Using a combination of biochemical and crystallographic methods we show that E. coli TldD and TldE interact to form a heterodimeric metalloprotease. TldD/E cleaves the N-terminal leader sequence from the modified MccB17 precursor peptide, to yield mature antibiotic, while it has no effect on the unmodified peptide. Both proteins are essential for the activity; however, only the TldD subunit forms a novel metal-containing active site within the hollow core of the heterodimer. Peptide substrates are bound in a sequence-independent manner through β sheet interactions with TldD and are likely cleaved via a thermolysin-type mechanism.

To explore the substrate binding site of the TldD/E heterodimer, wild-type or mutant (Glu263Ala) TldD/E was co-crystallized with a variety of peptides and peptide mimics, leading to four distinct ligand-bound complexes. Wild-type TldD/E crystals were grown in the presence of the peptide angiotensin II, and customized angiotensin II variant where the central (Tyr-Ile) peptide bond is replaced with a non-cleavable methylene bond, to yield two co-crystal structures with clear density for peptides where the carboxyl group of the C-terminal residue acts as a ligand to the catalytic zinc ion. However, the methylene bond variant gave density for a His-Pro-Phe peptide, i.e., the C-terminal portion of the added compound (hence WT-HPF); it was not clear whether the lack of clear density N-terminal to the His residue was due to a cleavage event, or simply that this region of the peptide was disordered. Using the standard nomenclature for protease active sites, these two ligands spanned subsites S4-S1 and S3-S1, respectively, occupying roughly half of the active site cleft.

>MGSSHHHHHHSQDPMSLNLVSEQLLAANGLKHQDLFAILGQLAERRLDYGDLYFQSSYHESWVLEDRIIKDGSYNIDQGVGVRAISGEKTGFAYADQISLLALEQSAQAARTIVRDSGDGKVQTLGAVEHSPLYTSVDPLQSMSREEKLDILRRVDKVAREADKRVQEVTASLSGVYELILVAATDGTLAADVRPLVRLSVSVLVEEDGKRERGASGGGGRFGYEFFLADLDGEVRADAWAKEAVRMALVNLSAVAAPAGTMPVVLGAGWPGVLLHEAVGHGLEGDFNRRGTSVFSGQVGELVASELCTVVDDGTMVDRRGSVAIDDEGTPGQYNVLIENGILKGYMQDKLNARLMGMTPTGNGRRESYAHLPMPRMTNTYMLPGKSTPQEIIESVEYGIYAPNFGGGQVDITSDKFVFSTSEAYLIENGKVTKPVKGATLIGSGIETMQQISMVGNDLKLDNGVGVCGKEGQSLPVGVGQPTLKVDNLTVGGTA[2x];>[2x]MALAMKVISQVEAQRKILEEAVSTALELASGKSDGAEVAVSKTTGISVSTRYGEVENVEFNSDGALGITVYHQNRKGSASSTDLSPQAIARTVQAALDIARYTSPDPCAGVADKELLAFDAPDLDLFHPAEVSPDEAIELAARAEQAALQADKRITNTEGGSFNSHYGVKVFGNSHGMLQGYCSTRHSLSSCVIAEENGDMERDYAYTIGRAMSDLQTPEWVGADCARRTLSRLSPRKLSTMKAPVIFANEVATGLFGHLVGAIAGGSVYRKSTFLLDSLGKQILPDWLTIEEHPHLLKGLASTPFDSEGVRTERRDIIKDGILTQWLLTSYSARKLGLKSTGHAGGIHNWRIAGQGLSFEQMLKEMGTGLVVTELMGQGVSAITGDYSRGAAGFWVENGEIQYPVSEITIAGNLKDMWRNIVTVGNDIETRSNIQCGSVLLPEMKIAGQ;>HPF[2x]5-(3,5-DICHLOROPHENYL)THIO-4-ISOPROPYL-1-(PYRIDIN-4-YL-METHYL)-1H-IMIDAZOL-2-YL-METHYL 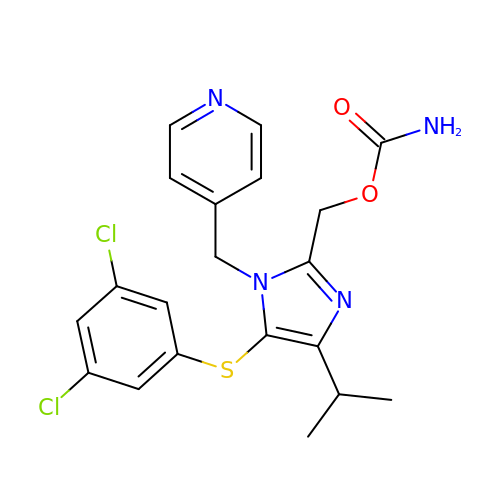CARBAMATE | C20 H20 Cl2 N4 O2 S | YQXCVAGCMNFUMQ-UHFFFAOYSA-N[(1~{R})-1-[2-[(5-azanyl-1,3,4-thiadiazol-2-yl)sulfanyl]ethanoylamino]-2-(4-carboxy-1,2,3-triazol-1-yl)ethyl]-$l^{3}-oxidanyl-bis(oxidanyl)boron | C9 H13 B N7 O6 S2 | 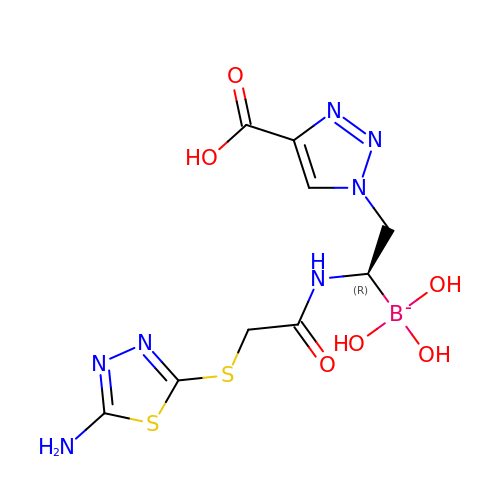QYCRGDXARHKIHF-YFKPBYRVSA-N>[3x]MISVGSNSNAFKEAVKSVKTILRNLTDGEITISAYDTAWVALIDAGDKTPAFPSAVKWIAENQLSDGSWGDAYLFSYHDRLINTLACVVALRSWNLFPHQCNKGITFFRENIGKLEDENDEHMPIGFEV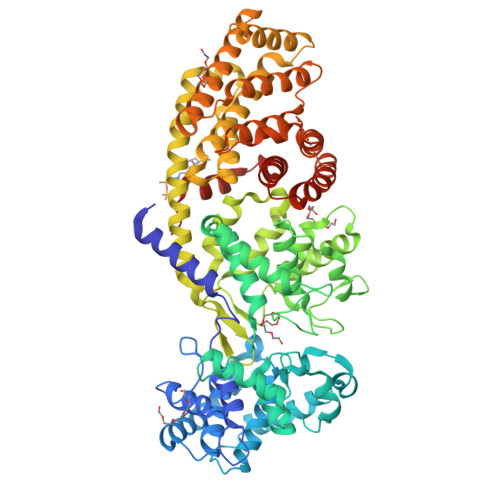AFPSLLEIARGINIDVPYDSPVLKDIYAKKELKLTRIPKEIMHKIPTTLLHSLEGMRDLDWEKLLKLQSQDGSFLFSPSSTAFAFMQTRDSNCLEYLRNAVKRFNGGVPNVFPVDLFEHIWIVDRLQRLGISRYFEEEIKECLDYVHRYWTDNGICWARCSHVQDIDDTAMAFRLLRQHGYQVSADVFKNFEKEGEFFCFVGQSNQAVTGMFNLYRASQLAFPREEILKNAKEFSYNYLLEKREREELIDKWIIMKDLPGEIGFALEIPWYASLPRVETRFYIDQYGGENDVWIGKTLYRMPYVNNNGYLELAKQDYNNCQAQHQLEWDIFQKWYEENRLSEWGVRRSELLECYYLAAATIFESERSHERMVWAKSSVLVKAISSSFGESSDSRRSFSDQFHEYIANARRSDHHFNDRNMRLDRPGSVQASRLAGVLIGTLNQMSFDLFMSHGRDVNNLLYLSWGDWMEKWKLYGDEGEGELMVKMIILMKNNDLTNFFTHTHFVRLAEIINRICLPRQYLKARRNDEKEKTIKSMEKEMGKMVELALSESDTFRDVSITFLDVAKAFYYFALCGDHLQTHISKVLFQKVGSHHHHHH>TELTKCKVSHAIKDIDGYQGISLLEWACVLFHTSGYDTQAVVNDNGSTEYGLFQISDRFWCKSSEFPESENICGISCDKLLDDELDDDIACAKKILAIKGIDYWKAYKPMCSEKLEQWRCEKP[2x];>[2x]ASMTGGQQMGRGSSLTACPEESPLLVGPMLIEFNIPVDLKLVEQQNPKVKLGGRYTPMDCISPHKVAIIIPFRNRQEHLKYWLYYLHPILQRQQLDYGIYVINQAGESMFNRAKLLNVGFKEALKDYDYNCFVFSDVDLIPMNDHNTYRCFSQPRHISVAMDKFGFSLPYVQYFGGVSALSKQQFLSINGFPNNYWGWGGEDDDIYNRLAFRGMSVSRPNAVIGKTRMIRHS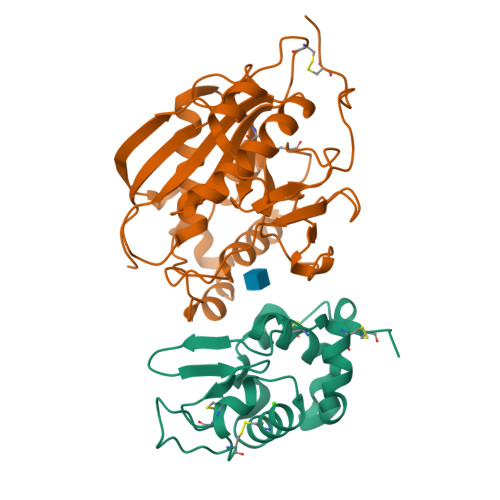RDKKNEPNPQRFDRIAHTKETMLSDGLNSLTYMVLEVQRYPLYTKITVDIGTPS>[2x]QDYGGTAAL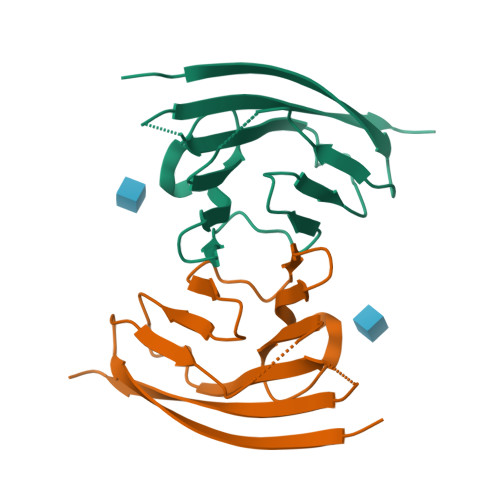LTSKEMRFSAAEGAKVLLSVPDQEENLLSFSWYKGKDVNENFTIAHYKKSSDSLQLGKKVSGREEIYKDGSMMLRAITLEDTGFYTLQTFKAHGQQEVTHVHLQVYKIVTKAENLYF>QIQLWQFLLELLSDSSNSSCITWEGTNGEFKMTDPDEVARRWGERKSKPNMNYDKLSRALRYYYDKNIMTKVHGKRYA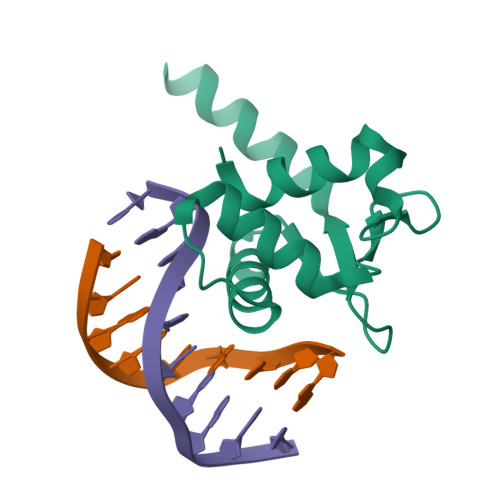YKFDFHGIAQALLEHHHHH[2x]>[3x]MVKQIESKTAFQEALDAAGDKLVVVDF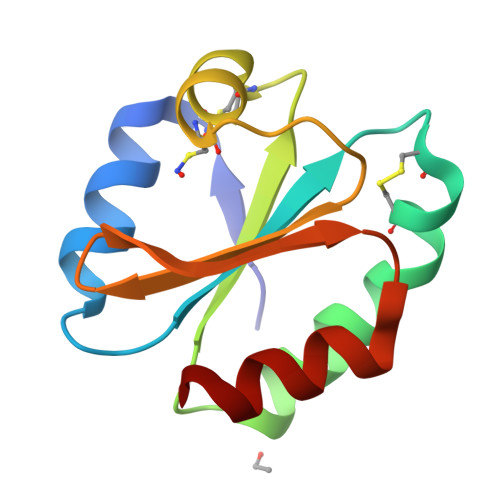SATWCGPCKMIKPFFHSLSEKYSNVIFLEVDVDDCQDVASECEVKCMPTFQFFKKGQKVGEFSGANKEKLEATINELV>SPLLKEQIETIVTGKKATVGVAVWGPDDLEPLLLNPFEKFPMQSVFKLHLAMLVLHQVDQGKLDLNQSVTVNRAA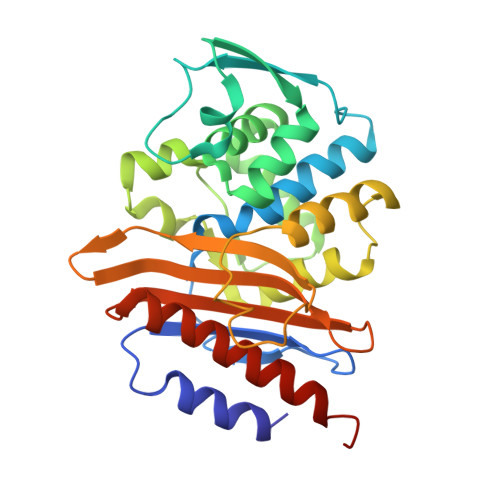VLQNTWSPMMKDHQGDEFTVAVQQLLQYSVSHSDNVACDLLFELVGGPQALHAYIQSLGVKEAAVVANEAQMHADDQVQYQNWTSMKAAAQVLQKFEQKKQLSETSQALLWKWMVETTTGPQRLKGLLPAGTIVAHKTGTSGVRAGKTAATNDAGVIMLPDGRPLLVAVFVKDSAESERTNEAIIAQVAQAAYQFELKKLSAVSPD[4x]> MKLHTDPATALNTV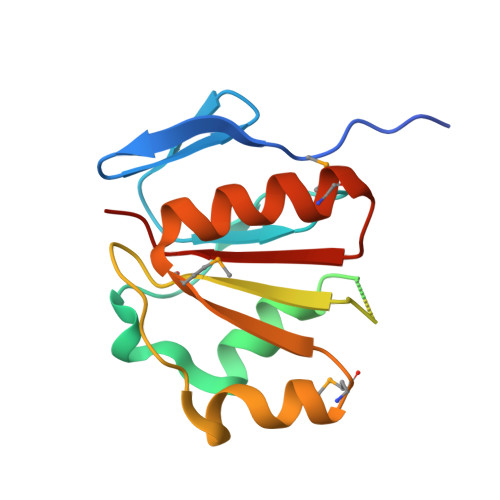TAYGDGYIEVNQVRFSHAIAFAPEGPVASWPVQRPADITASLLQQAAGLAEVVRDPLAFLDEPEAGAGARPANAPEVLLVGTGRRQHLLGPEQVRPLLAMGVGVEAMDTQAAARTYNILMAEGRRVVVALLPDGDS A HEPN (higher eukaryote and prokaryote nucleotide binding) nuclease Las1 and a polynucleotide kinase Grc3 assemble into a tetramerase responsible for rRNA maturation. Las1 and Grc3 are highly conserved proteins and have recently been identified as core enzymes involved in processing and removing ITS2 spacer, which is a key step in the synthesis of 60S ribosomal subunit. Recent studies have demonstrated that Las1 is an endoribonuclease that contains a HEPN (higher eukaryote and prokaryote nucleotide binding) domain responsible for rRNA processing. Grc3 is a polynucleotide kinase responsible not only for Las1 nuclease activation, but also for nonspecific phosphorylation of the 5′-OH of the 26S pre-rRNA produced by Las1 cleavage, providing a signal for further processing by Rat1-Rai1 exonuclease.

To elucidate how Las1 and Grc3 cooperate to direct ITS2 cleavage and phosphorylation, we determined the cryo-EM and crystal structures of full-length ScLas1-Grc3 complex at 3.07 Å and 3.69 Å resolution, respectively. To be noted, the crystal structures were solved by molecular replacement method with the cryo-EM maps of Las1-Grc3 complexes. Each Grc3 GCT binds to a groove in each Las1 HEPN domain and extends to the ribonuclease active center, which is formed by the two HEPN domains via dimerization. Both the crystal and cryo-EM structures show that the conserved catalytic residues Arg129, His130, His134 with two copies from two HEPN domains form a symmetric catalytic active pocket. Our crystal and cryo-EM structures exhibit that the Las1 LCT is located in a groove in the CTD domain of Grc3. Notably, compared with CjGrc3-bound CjLas1, ScGrc3-bound ScLas1 has a more compact catalytic pocket, which may explain why ScLas1 shows better ITS2 cleavage activity than CjLas1 in the presence of Grc3. In addition, His130 in the ScLas1-Grc3 complex active site and the analogous His130 in the CjLas1-Grc3 complex active site adopt two different conformations, which are similar to the conformations of His142 of CtGrc3-bound CtLas1 in two different active states.

>MVIDSKQDLPQYTKDSGSESDSDSSNNFIVESPSIPSSKSATVVLNSEEYEDDEGDDLNGLDAELIDNITYEGDEDETMFVGLKEKQKLHLSGVFRLQVVKGGIVYNNVHYNASREILTFWHPLSQSIPTIDFSHFAGWQDTFFMPRNNRFKIRDEEFKSFPCVLRVFNSNHTGLLEAGHLYRDVNYLWKPKEPYFPLNERTTYHLLHESDRIQSLSVPGYWSTPLEKLYLSHKNAAYDTRIMVIGGKNSGKSTFLRLLLEKFTQDIRDSTTSQEELVYLDLDPGQPEYSLPDSISLNKILSSPISLGQHLCQGSNFQTLLQFYAGSSSPQDEPTSYLNCADKLIDHLEEQAFFGTSLLNLPGWIKGFGMQILNHIIRKYKPTHLLFLETANSKRHLDELTIPQSFSTSLRDAYAPEVVRVPAHSLNHTLSSRFHASQLRTFKILALFHKITQFDYDFAPLLKSAPLQISYGKGKSGIKGIQFPMEFQDLNPQDIKSALEGTVIGIYTYSGEDSLEVKSLNTFPILQSCTSSSKNFITLGLIHSIDTSQQIMNIYVPPCHTQILDKQPEDAQWIIVRNKTETPFCDFLPSPRTITWDDNIQIPFATFERRKKLEHVWKVRKNVMRRGQFMKR[2x];>[2x]MIPPRIVPWRDFAELEELKLWFYPKSKGTIEDKRQRAVQRVQSYRLKGSQYLPHVVDSTAQITCAVLLDEKEACLGVHQDSIPIRLSYVMALIRFVNGLLDPTQQSQFAIPLHTLAAKIGLPSWFVDLRHWGTHERDLPGLEMLRWAANEALSWLYDHYWNDEELEDDRDDDDDDDDTGYGYRRNDKLEKYMESLTKTLDKWKRLRNEFLEYKWVWENANDSLITSSNFSGDNLVNYDAEKRKSSHASSSETMIRENLRQWQELWKLSIYHNVVLEKFFNNYDPLLLKVLMLNLNNFDWKVIEWVARNYRTQQDDSNITTILKRKFNAWKELQKRLLDVIINNLNNKNFKNKWQNWEKLIDENASYLILYFCQSMLAKLETEKITGNSWRNKKRRKQIDSTVEIEAKLKENIDNLSLRFNEGEIKLYDFIPAEKDSVPLKKEVSPALKADTNDILGDLASLKQRMSSFGTVGKKNKQEENRATPVKNWSRVQNWKPKPFGVL> MALTGCSEKININEDKISHKIDIPDSAWTIGIGEKFKNAGHPNVKYPMIDDSYVQGAPLGGFGAGTIGRTYNGGFSRWHLEIGKNKYTTVYANQFSVFQKVEGNKDGVAQVLYAGEPENGYLSS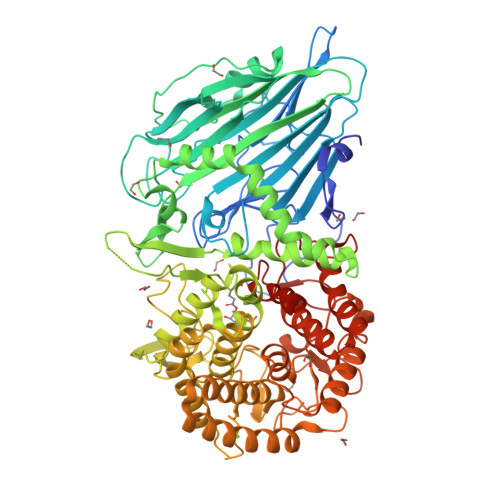WKWDYPKESGMYYALYPNSWYTYTNKDLPVQLAVKQFSPIIPYNYKETSYPVAVFKWTAYNPTNKNVDVSIMFTWQNMIGFFGKQVNVNSGNFNKIIKDKSKDSEIVAAVMGNISNDNEEWNGEYSIGVKKVPGVDISYKAKFVTTGDGSDLWHEFSKNGILDNKDDETPTKQDGIGSAIAVNFKLQPGQTIEVPFALSWDLPIMKFGGGDKWYKMYTKYFGKNGKNSFAILKEALNNYQKWEKMIDDWQKPILSNKSKPDWYKTALFNELYYLADGGTAWENGKVGEKDKRTNNMFGLLECFDYNYYETLDVRFYGSFPLVMLWPDIEKQVMRQFADTINVQDSSEFKVGSNGAMAVKKVQGMIPHDLGSSYALPWIKINAYDWQNPNIWKDLNSKYVLLVYRDYVLTGKTDKEFLKYTWKSVKTALDKLKEMDKDNDGIPDNEGIPDQTYDTWSMKGTSAYCGSLWLAALKAAQEIGKVLKDNEAYIKYNEWYKIAQQNFEKELWNGEYYNFDTESDHKDSIMADQLAGQWYADILRLGDILPKDHVQKALKKIYEFNVMKFENGKMGAVNGMRPDGIVDESDIQAQEVWTGVTYALASFMKYRGMTEEAYNTAYGVYKMTYDKSGKGYWFRTPEAWTKDGNYRASMYMRPLSIWSMEVNYNEVLEHHHHHH>[2x]DDSLPDLKIEKLEKGVYVHTSFEEVKGWGV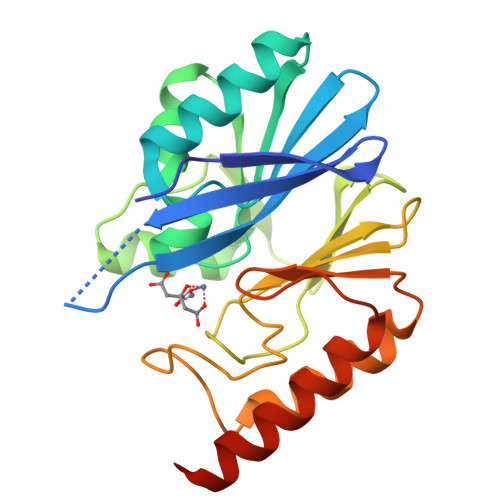VTKHGLVVLVKNDAYLIDTPITAKDTEKLVNWFIEHGYRIKGSISTHFHGDSTAGIEWLNSQSISTYASELTNELLKKDNKVQATNSFSGVSYSLIKNKIEVFYPGPGHTQDNVVVWLPEKKILFGGCFVKPDGLGNLGDANLEAWPKSAKILMSKYGKAKLVVSSHSEIGNASLLQRTWEQAVKGLNESKKPLQPSS>GGRDKDHLLKYNVGDLVWSKVSGYPWWPCMVSADPLLHSYTKLKGQKKSARQYHVQFFGDAPE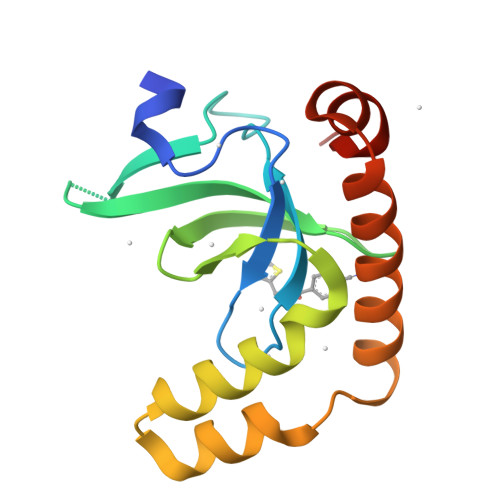RAWIFEKSLVAFEGEGQFEKLCQESAKQAPTKAEKIKLLKPISGKLRAQWEMGIVQAEEAASMSVEERKAKFTFLYVG[8x]>MASTRCKLARYLEDLEDVDLKKFKMHLEDYPPQKGCIPLPRGQTEKADHVDLATLMIDFNGEEKAWAMAVWIFAAINRRDL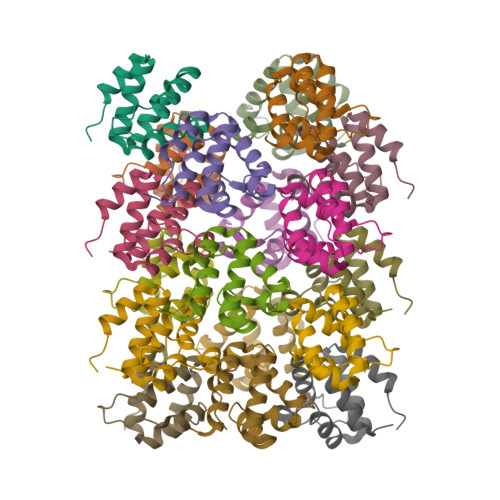YEKAKRDEPKWGSDNARVSNPTVISQE[18x]> GSGAMAQNLDSMLHGTGMKSDSDQKKSEN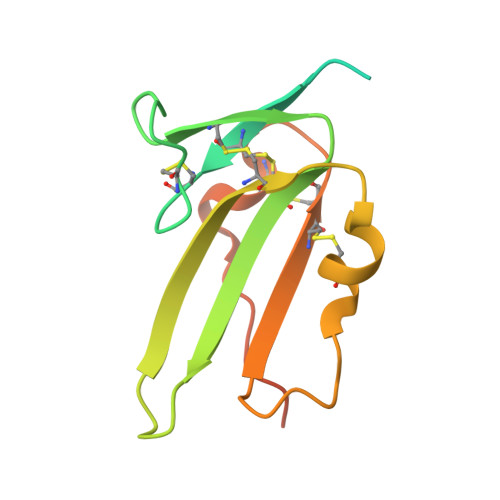GVTLAPEDTLPFLKCYCSGHCPDDAINNTCITNGHCFAIIEEDDQGETTLASGCMKYEGSDFQCKDSPKAQLRRTIECCRTNLCNQYLQPTLPPVVIGPFFDGSIR>MGMQGDPDVLRLLNEQLTSELTAINQYFLHSKMQDNWGFTELAAHTRAESFDEMRHAEEITDRILLLDGLPNYQRIGSLRIGQTLREQFEADLAIEYDVLNRLKPGIVMCREKQDTTSAVLLEKIVA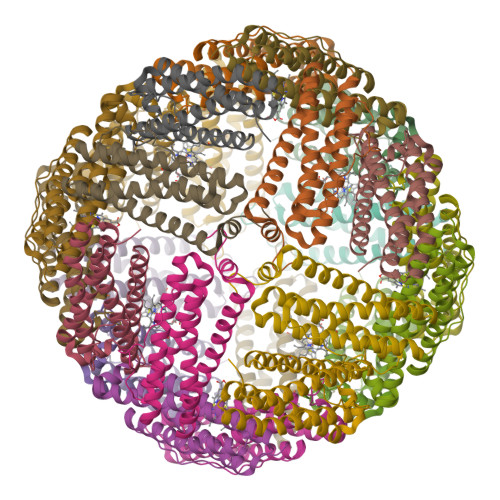DEEEHIDYLETQLELMDKLGEELYSAQCVSRPPTKLAAALEHHHHHH[6x]> MDPDQYSIEADKKFKYSVKLSDYPTLQDAASAAVDGLLIDRDYNFYGGETVDFGGKVLTIECKAKFIGDGNLIFTKLGKGSRIAGVFMESTTTPWVIKPWTDDNQWLTDAAAVVATLKQSKTD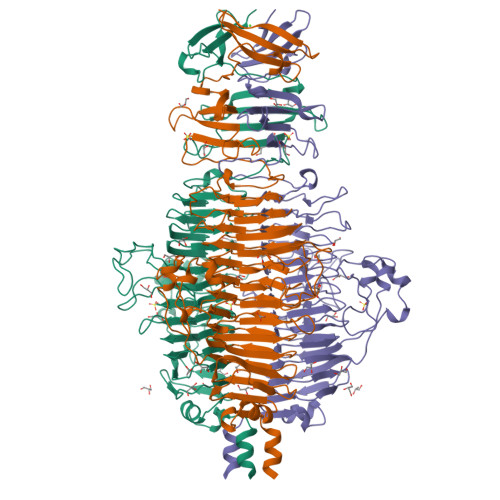GYQPTVSDYVKFPGIETLLPPNAKGQNITSTLEIRECIGVEVHRASGLMAGFLFRGCHFCKMVDANNPSGGKDGIITFENLSGDWGKGNYVIGGRTSYGSVSSAQFLRNNGGFERDGGVIGFTSYRAGESGVKTWQGTVGSTTSRNYNLQFRDSVVIYPVWDGFDLGADTDMNPELDRPGDYPITQYPLHQLPLNHLIDNLLVRGALGVGFGMDGKGMYVSNITVEDCAGSGAYLLTHESVFTNIAIIDTNTKDFQANQIYISGACRVNGLRLIGIRSTDGQSLTIDAPNSTVSGITGMVDPSRINVANLAEEGLGNIRANSFGYDSAAIKLRIHKLSKTLDSGALYSHINGGAGSGSAYTQLTAISGSTPDAVSLKVNHKDCRGAEIPFVPDIASDDFIKDSSCFLPYWENNSTSLKALVKKPNGELVRLTLATL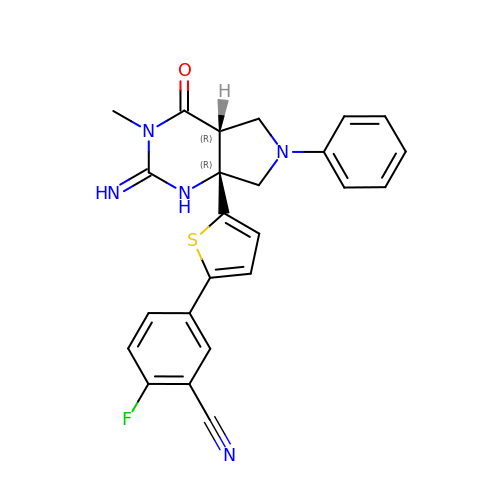2-fluoro-5-{5-[(2E,4aR,7aR)-2-imino-3-methyl-4-oxo-6-phenyloctahydro-7aH-pyrrolo[3,4-d]pyrimidin-7a-yl]thiophen-2-yl}benzonitrile | C24 H20 F N5 O S | DWVJKKOFIHHAKC-UUOWRZLLSA-N>MGHHHHHHENLYFQGVQKIGILGAMREEITPILELFGVDFEEIPLGGNVFHKGVYHNKEIIVAYSKIGKVHSTLTTTSMILAFGVQKVLFSGVAGSLVKDLKINDLLVATQLVQHDVDLSAFDHPLGFIPESAIF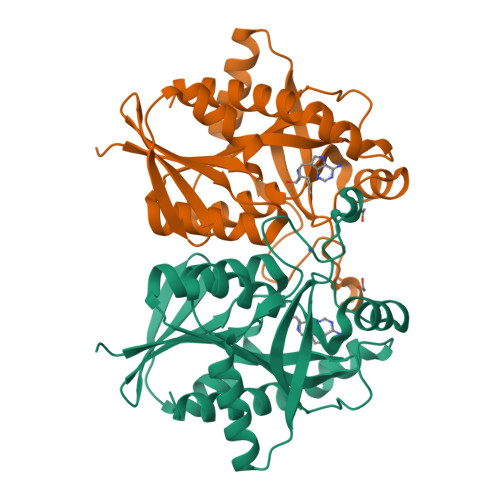IETSGSLNALAKKIANEQHIALKEGVIASGDQFVHSKERKEFLVSEFKASAVEMEGASVAFVCQKFGVPCCVLRSISDNADEKAGMSFDEFLEKSAHTSAKFLKSMVDEL[2x]>MKNKVVVVTGVPGVGGTTLTQKTIEKLKEEGIEYKMVNFGTVMFEVAKEEGLVEDRDQMRKLDPDTQKRIQKLAGRKIAEMAKESNVIVDTHSTVKTPKGYLAGLPIWVLEELNPDIIVIVETSSDEILMR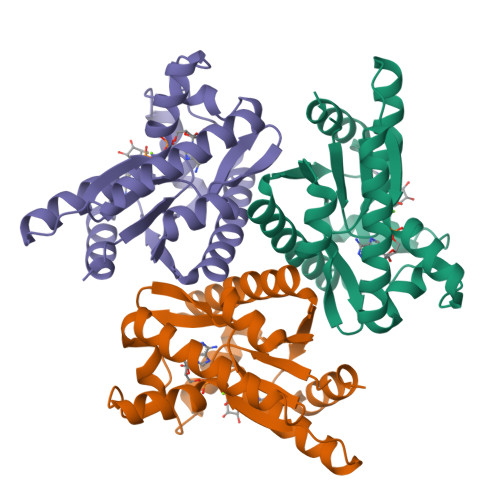RLGDATRNRDIELTSDIDEHQFMNRCAAMAYGVLTGATVKIIKNRDGLLDKAVEELISVLKLEHHHHHH[12x]> MAGMALARAWKQMSWFYYQYLLVTALYMLEPWERTVFNSMLVSIVGMALYTGYVFMPQHIMAI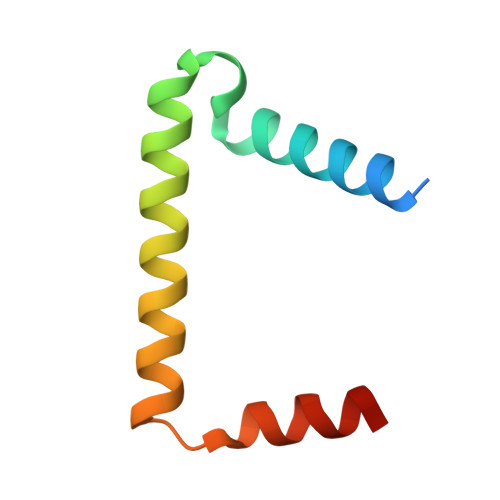LHYFEIVQ>MSKPSIVILGAGYGGIVAALGLQKRLNYNEADITLVNKNDYHYITTELHQPAAGTMHHDQARVGIKELIDEKKIKFVKDTVVAIDREQQKVTLQNGELHYDYLVVGLGSEPETFGIEGLREHAFSINSINSVRIIRQHIEYQFAKFAAEPERTDYLTIVVGGAGFTGIEFVGELADRMPELCAEYDVDPKLVRIINVEAAPTVLPGFDPALVNYAMDVLGGKGVEFKIGTPIKRCTPEGVVIEVDGEEEEIKAATVVWTGGVRGNSIVEKSGFETMRGRIKVDPYLRAPGHENIFIVGDCALIINEENNRPYPPTAQIAIQHGENVAANLAALIRGGSMTPFKPHIRGTVASLGRNDAIGIVGGRKVYGHAASWLKKLEDMRYLYLIGGLSLVLKKGRFHHHHHH[4x]

Type-II NADH:quinone oxidoreductase (NADH dehydrogenase-2, NDH-2) is a membrane-bound dehydrogenase that oxidizes NADH and reduces quinones and is a central feature of the respiratory chain in many diverse species, but not in animals. NDH-2 is also much smaller and simpler in structure than complex I – it comprises only a single subunit and one flavin redox cofactor. All of them are homodimers, with each monomer containing two Rossmann folds that form nucleotide-binding sites for a noncovalently bound flavin adenine dinucleotide (FAD) and the NADH substrate. Our study has revealed how the NADH:quinone oxidoreduction reaction proceeds in two half reactions (NADH oxidation + reduction of the flavin, and re-oxidation of the flavin + reduction of quinone) that occur independently of each other and use spatially distinct substrate-binding sites.

To test the proposal that the two substrate reactions are independent of each other we mutated a key residue in each substrate-binding site. G164 is positioned next to the adenine-proximal ribose of the bound nucleotide and I379 is positioned at the entry to the quinone-binding pocket. Structures of the two mutants, at 3.2 and 2.7 Å resolution, respectively, confirmed that the structural changes are localized and the integrities of the structures are maintained. On the other hand, I379E crystallized in the same space group as the WT and the side chain was observed in three of four molecules in the asymmetric unit. In comparison with WT, G164E and I379E exhibit RMSD values of 0.54 Å (Cα of 395 residues) and 0.45 Å (Cα of 393 residues), respectively, with no substantial additional differences. For the I379E variant, the KM for menadione increases significantly, to 780 μM, consistent with the mutation compromising quinone binding. Again, the observed rates are lower, with the maximal rate equivalent to ~60% of the WT rate, and, as expected, the apparent KM value for NADH has decreased. When oxidized I379E reacts with NADH, the flavin is reduced and a CTC forms, as in the WT enzyme. As in the WT enzyme the reaction with NADH is rapid (~290 s−1 in 2 μM NADH), but when the NADH-reduced enzyme is exposed to menadione the reaction is very slow (~3 s−1 in 1.5 μM menadione). Therefore, in the I379E variant the menadione reaction is compromised but, irrespective of the functionality of the quinone-binding site, the NADH-binding site functions properly.Previous studies showed that proper introduction of disulfide bonds could stabilize the flexible region of target proteins and reduce the conformational entropy by locking the protein into single desired conformation. Here we developed a comprehensive disulfide bond prediction algorithm that not just increased the success rate of predictions but also improved the quality of crystallized target proteins. We applied our method on two proteins which were previously determined to high resolution and frequently used as fusion partners for GPCR crystallization, cytochrome b562 (BRIL) and Flavodoxin, and verified our prediction by solving the crystal structures of the wild type (WT) proteins and mutants. The theoretical and experimental results both indicated that with relatively lower values of conformational entropy, proteins would be more stable and readily crystallized to higher diffraction resolution.

Eventually, four pairs of BRIL mutants and three pairs of Flavodoxin mutants, together with their WT proteins, were crystallized and structure determined. The WT and disulfide engineered Flavodoxin structures were determined to high-resolution of 1.20–1.55 Å with B-factors in the range of 16.15–19.24 Å2. Based on our algorithm, the best-engineered constructs of BRIL and Flavodoxin show lower entropy and higher diffraction quality than the wild type proteins, and the predicted disulfide bond on GLP-1R facilitated crystallization of the GLP-1R transmembrane domain.

> SAKALIVYGSTTGNTEYTAETIARELADAGYEVDSRDAASVEAGGLFEGFDLVLLGCSTWGDDSIELQDDFIPLFDSLEETGAQGRKVACFGCGDSSWEYFCGAVDAIEEKLKNLGAEIVQDGLRIDGDPRAARDDIVGWAHDVRGAI>[2x]GHHHHHHAMSMQDTLLTLDTPAAVIDLDRMQ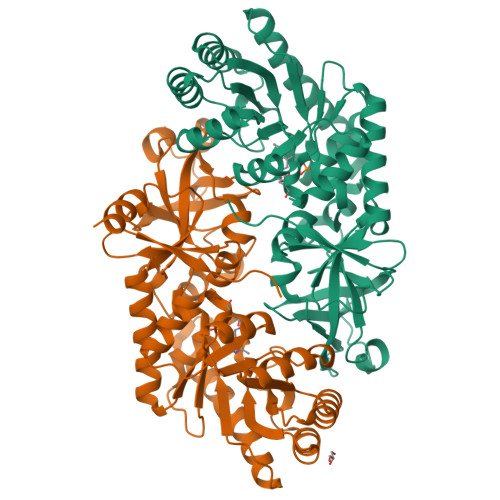RNIARMQQRMDAQGVRLRPHVKTSKSVPVAAAQRAAGASGITVSTLKEAEQFFAAGTTDILYAVSMAPHRLPQALQLRRRGCDLKLIVDSVAAAQAIAAFGREQGEAFEVWIEIDTDGHRSGVGADDTPLLLAIGRTLHDGGMRLGGVLTHAGSSYELDTPEALQALAERERAGCVQAAEALRAAGLPCPVVSVGSTPTALAASRLDGVTEVRAGVYVFFDLVMRNIGVCAAEDVALSVLATVIGHQADKGWAIVDAGWMAMSRDRGTARQKQDFGYGQVCDLQGRVMPGFVLTGANQEHGILARADGAAEADIATRFPLGTRLRILPNHAAATGAQFPAYQALAADGSVQTWERLHGW> SMQTTNIRKTFIFMEVLGSGAFSEVFLVKQRLTGKLFALKCIKKSPAFRDSSLENEIAVLKKIKHENIVTLEDIYESTTHYYLVMQLVSGGELFDRILERGVYTEKDASLVIQQVLSAVKYLHENGIVHRDLKPENLLYLTPEENSKIMITDFGLSKMEQNGIMSTACGTPGYVAPEVLAQKPYS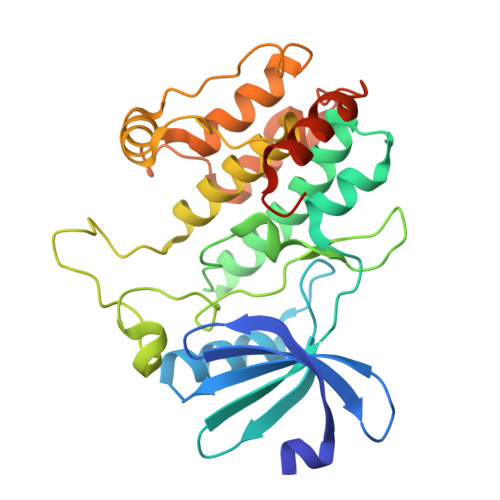KAVDCWSIGVITYILLCGYPPFYEETESKLFEKIKEGYYEFESPFWDDISESAKDFICHLLEKDPNERYTCEKALSHPWIDGNTALHRDIYPSVSLQIQKNFAKSKWRQAFNAAAVVHH3,3'-dimethoxybiphenyl-4,4'-diamine | C14 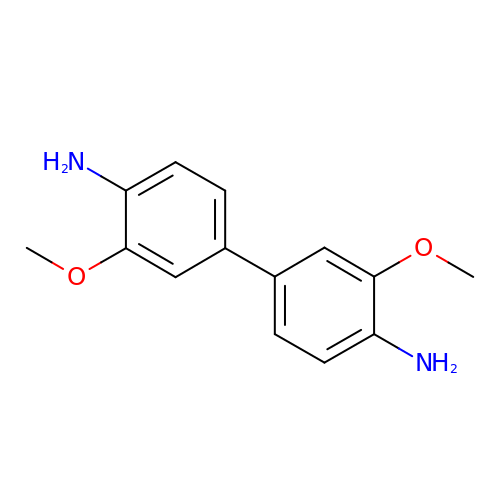H16 N2 O2 | JRBJSXQPQWSCCF-UHFFFAOYSA-N>STFVAKDGTQIYFKDWGSGKPVLFSHGWILDADMWEYQMEYLSSRGYRTIAFDRRGFGRSDQPWTGNDYDTFADDIAQLIEHLDLKEVTLVGFSMGGGDVARYIARHGSARVAGLVLLGAVTPLFGQKPDYPQGVPLDVFARFKTELLKDRAQFISDFNAPFYGINKGQVVSQGVQTQTLQIALLASLKATVDCVTAFAETDFRPDMAKIDVPTLVIHGDGDQIVPFETTGKVAAELIKGAELKVYKDAPHGFAVT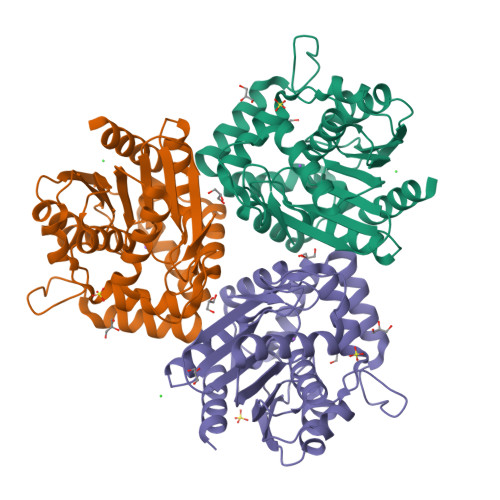HAQQLNEDLLAFLKR[6x]>[2x]MYGKIIFVLLLSEIVSISASSTTGVAMHTSTSSSVTKSYISSQTNDTHKRDTYAATPRAHEVSEISVRTVYPPEEETGER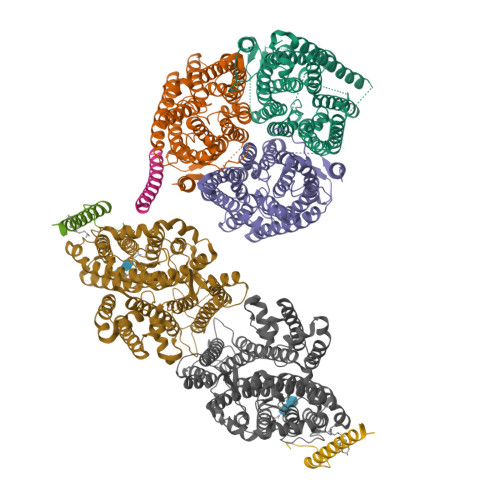VQLAHHFSEPEITLIIFGVMAGVIGTILLISYGIRRLIKKSPSDVKPLPSPDTDVPLSSVEIENPETSDQ;>MEELQDDYEDMMEENLEQEEYEDPDIPESQMEEPAAHDTEATATDYHTTSHPGTHKVYVELQELVMDEKNQELRWMEAARWVQLEENLGENGAWGRPHLSHLTFWSLLELRRVFTKGTVLLDLQETSLAGVANQLLDRFIFEDQIRPQDREELLRALLLKHSHAGELEALGGVKPAVLTRSGDPSQPLLPQHSSLETQLFCEQGDGGTEGHSPSGILEKIPPDSEATLVLVGRADFLEQPVLGFVRLQEAAELEAVELPVPIRFLFVLLGPEAPHIDYTQLGRAAATLMSERVFRIDAYMAQSRGELLHSLEGFLDCSLVLPPTDAPSEQALLSLVPVQRELLRRRYQSSPAKPDSSFYKGLDLNGGPDDPLQQTGQLFGGLVRDIRRRYPYYLSDITDAFSPQVLAAVIFIYFAALSPAITFGGLLGEKTRNQMGVSELLISTAVQGILFALLGAQPLLVVGFSGPLLVFEEAFFSFCETNGLEYIVGRVWIGFWLILLVVLVVAFEGSFLVRFISRYTQEIFSFLISLIFIYETFSKLIKIFQDHPLQKTYNYNVLMVPKPQGPLPNTALLSLVLMAGTFFFAMMLRKFKNSSYFPGKLRRVIGDFGVPISILIMVLVDFFIQDTYTQKLSVPDGFKVSNSSARGWVIHPLGLRSEFPIWMMFASALPALLVFILIFLESQITTLIVSKPERKMVKGSGFHLDLLLVVGMGGVAALFGMPWLSATTVRSVTHANALTVMGKASTPGAAAQIQEVKEQRISGLLVAVLVGLSILMEPILSRIPLAVLFGIFLYMGVTSLSGIQLFDRILLLFKPPKYHPDVPYVKRVKTWRMHLFTGIQIICLAVLWVVKSTPASLALPFVLILTVPLRRVLLPLIFRNVELQCLDADDAKATFDEEEGRDEYDEVAMPV[2x];> MSSKYPRSVRRCLPLWALTLEAALILLFYFFTHYDASLEDQKGLVASYQVGQDLTVMAALGLGFLTSNFRRHSWSSVAFNLFMLALGVQWAILLDGFLSQFPPGKVVITLFSIRLATMSAMSVLISAGAVLGKVNLAQLVVMVLVEVTALGTLRMVISNIFNTDYHMNLRHFYVFAAYFGLTVAWCLPKPLPKGTEDNDQRATIPSLSAMLGALFLWMFWPSVNSPLLRSPIQRKNAMFNTYYALAVSVVTAISGSSLAHPQRKISMTYVHSAVLAGGVAVGTSCHLIPSPWLAMVLGLVAGLISIGGAKCLPVCCNRVLGIHHISVMHSIFSLLGLLGEITYIVLLVLHTVWNGNGMIGFQVLLSIGELSLAIVIALTSGLLTGLLLNLKIWKAPHVAKYFDDQVFWKFPHLAVGF;>[2x]MRFTFPLMAIVLEIAMIVLFGLFVEYETDQTVLEQLNITKPTDMGIFFELYPLFQDVHVMIFVGFGFLMTFLKKYGFSSVGINLLVAALGLQWGTIVQGILQSQGQKFNIGIKNMINADFSAATVLISFGAVLGKTSPTQMLIMTILEIVFFAHNEYLVSEIFKASDIGASMTIHAFGAYFGLAVAGILYRSGLRKGHENEESAYYSDLFAMIGTLFLWMFWPSFNSAIAEPGDKQCRAIVNTYFSLAACVLTAFAFSSLVEHRGKLNMVHIQNATLAGGVAVGTCADMAIHPFGSMIIGSIAGMVSVLGYKFLTPLFTTKLRIHDTCGVHNLHGLPGVVGGLAGIVAVAMGASNTSMAMQAAALGSSIGTAVVGGLMTGLILKLPLWGQPSDQNCYDDSVYWKVPKTR;> MYGKIIFVLLLSEIVSISALSTTEVAMHTSTSSSVTKSYISSQTNGETGQLVHRFTVPAPVVIILIILCVMAGIIGTILLISYSIRRLIKA> MIIIRYLVRETLKSQLAILFILLLIFFCQKLVKILGAAVDGEIPTNLVLSLLGLGIPEMAQLILPLSLFLGLLMTLGKLYTESEITVMHACGLSKAVLVKAAMILALFTGIVAAVNVMWAGPMSSRHQDEVLAEAKANPGMAALAQGQFQQATDGNSVLFIESVDGSKFNDVFLAQLRTKGNARPSVVVADSGQLAQRKDGSQVVTLNKGTRFEGTAMLRDFRITDFQNYQAIIGHQAVALDPTDTEQMDMRTLWNTDTDRARAEFHWRITLVF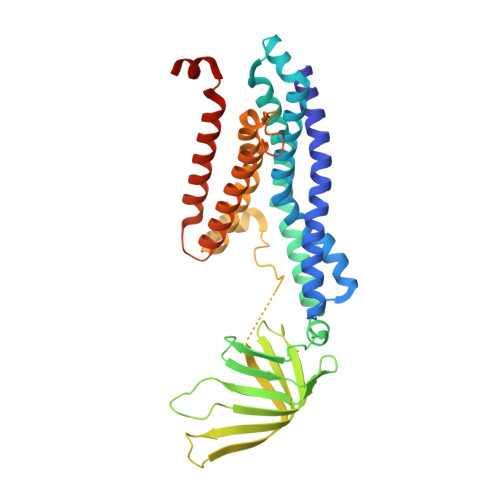TVFMMALIVVPLSVVNPRQGRVLSMLPAMLLYLIYFLLQTSIRSNGAKGKLDPMVWTWFVNSLYILLALGLNLWDTVPVRRIRARFSRKGAI>[6x]MGFLKGKKGLIVGVANNKSIAYGIAQSCFNQGATLAFTYLNESLEKRVRPIAQELNSPYVYELDVSKEEHFKPLYDSVKKDLGSLDFIVHSVAFAPKEALEGSLLETSKSAFNTAMEISVYSLIELTNTLKPLLNNGASVLTLSYLGSTKYMAHYNVMGLAKAALESAVRYLAVDLGKHNIRVNALSAGPIRTLASSGIADFRMILKWNEINAPLRKNVSLEEVGNAGMYLLSSLSSG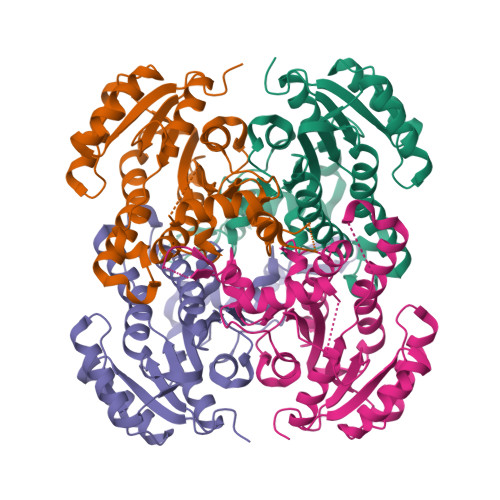VSGEVHFVDAGYHVMGMGAVEEKDNKATLLWDLHKEQ> MRGSHHHHHHGSASF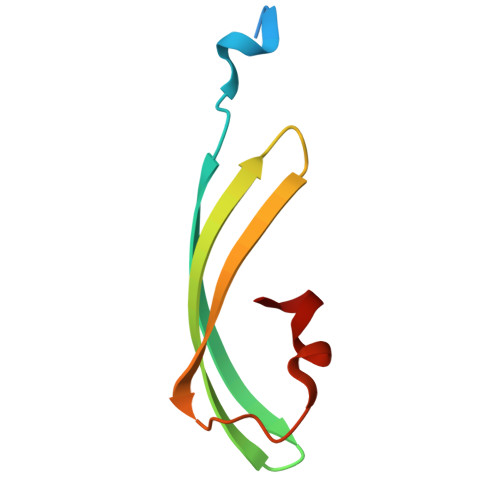LKKTMPFKTTIEGTVNGHYFKCTGKGEGNPFEGTQEMKIEVIEGGPLPFAFHILSTSC6-(4-{[3-(3,5-dichloropyridin-4-yl)-5-(1-methylethyl)isoxazol-4-yl]methoxy}-2-methylphenyl)-1-methyl-1H-indole-3-carboxylic 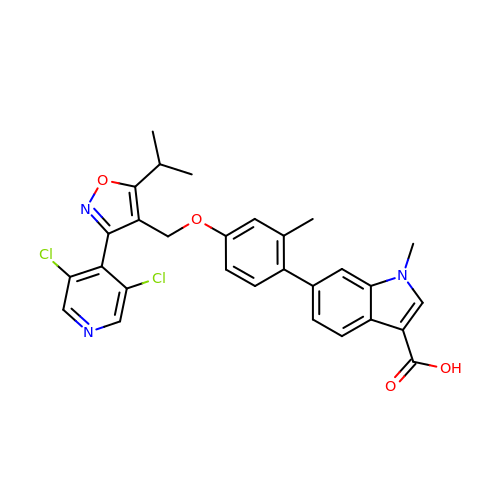acid | C29 H25 Cl2 N3 O4 | JTRRVYQZHXAOGI-UHFFFAOYSA-N> MRGSHHH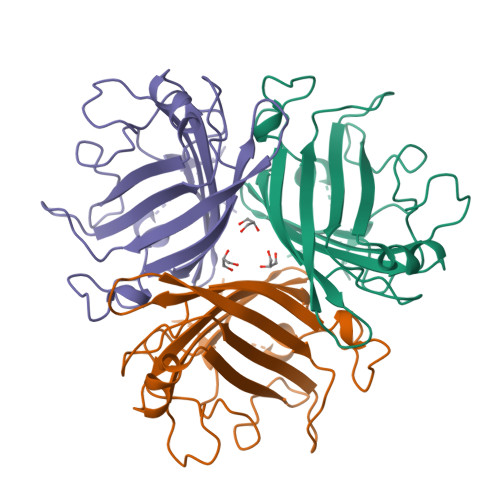HHHGSGDICIKDSINTLWTGINPPPNCQIVENTNTNDGKLTLVLVKNGGLVNGYVSLVGVSDTVNQMFTQKTANIQLRLYFDSSGNLLTEESDLKIPLKNKSSTATSETVASSKAFMPSTTAYPFNTTTRDSENYIHGICYYMTSYDRSLFPLNISIMLNSRMISSNVAYAIQFEWNLNASESPESNIATLTTSPFFFSYITEDDN>[2x]GSMALLTAETFRLQFNNRRRLRRPYYPRKALLCYQLTPQNGSTPTRGYFENKKKCHAEICFINEIKSMGLDETQCYQVTCYLTWS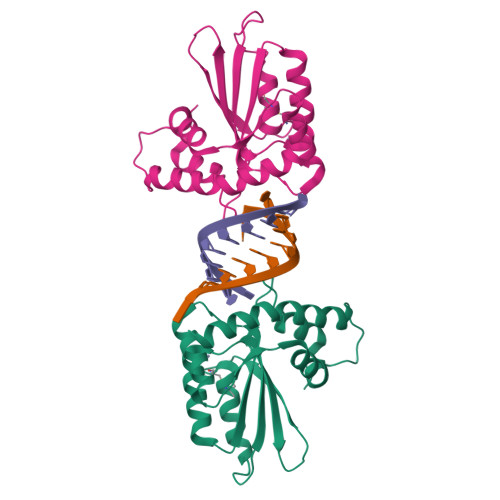PCSSCAWKLVDFIQAHDHLNLRIFASRLYYHWCKPQQEGLRLLCGSQVPVEVMGLPEFNDCWENFVDHEKPLSFDPCKMLEELDKNSRAIKRRLERIKQS>MKYMITSKGDEKSDLLRLNMIAGFGEYDMEYDDVEPEIVISIGGDGTFLSAFHQYEERLDEIAFIGIHTGHLGFYADWRPAEADKLVKLLAKGEYQKVSYPLLKTTVKYGIGKKEATYLALNESTVKSSGGPFVVDVVINDIHFERFRGDGLCMSTPSGTTAYNKSLGGALMHPSIEAMQLTEMASINNRVYRTIGSPLVFPKHHVVSLQPVNDKDFQISVDHLSILHRDVQEIRYEVSAKKIHFARFRSFPFWRRVHDSF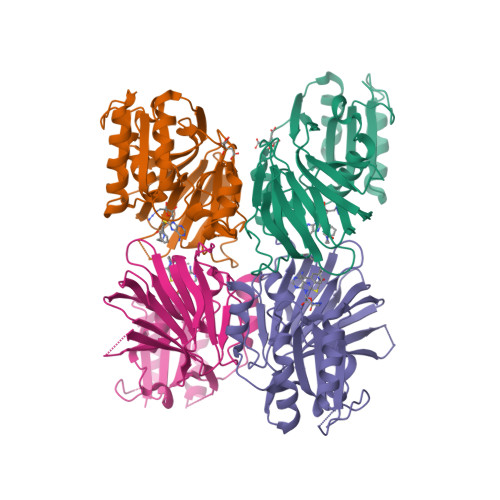IEDLEHHHHHH[4x]> GHSSSDP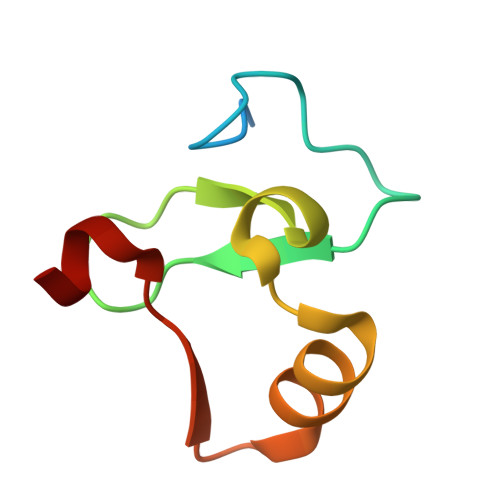VYPCGICTNEVNDDQDAILCEASCQKWFHRICTGMTETAYGLLTAEASAVWGCDTCMA> AAQPAEALEDDGLCSADQKSCAQSEPDQINEDEFSFKIRRQIEKANADYKPCSSDPQDSDCSCHANVLKRDLAPYKSTGVTRQMIESSARYGTKYKIYGHRLYRDANCMFPARCEGIEHFLLPLVATLPDMDLIINTRDYPQLNAAWGNAAGGPVFSFSKTKEYRDIMYPAWTF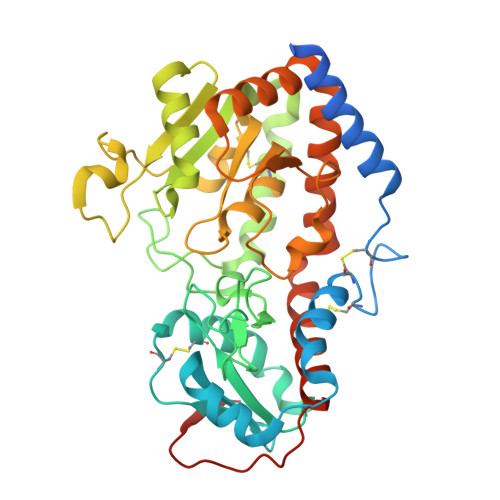WAGGPATKLHPRGIGRWDQMREKLEKRAAAIPWSQKRSLGFFRGSRTSDERDSLILLSRRNPELVEAQYTKNQGWKSPKDTLDAPAADEVSFEDHCKYKYLFNFRGVAASFRLKHLFLCKSLVFHVGDEWQEFFYDQLKPWVHYVPLKSYPSQQEYEHILSFFKKNDALAQEIAQRGYDFIWEHLRMKDIKCYWRKLLKRYVKLLQYEVKPEDQLIYIGPKARALVPR>MHHHHHHGSDDDDKRPEAKSAQPADGWKGERPRSEEDNELNLPNLAAAYSSILSSLGENPQRQGLLKTPWRAASAMQFFTKGYQETISDVLNDAIFDEDHDEMVIVKDIDMFSMCEHHLVPFVGKVHIGYLPNKQ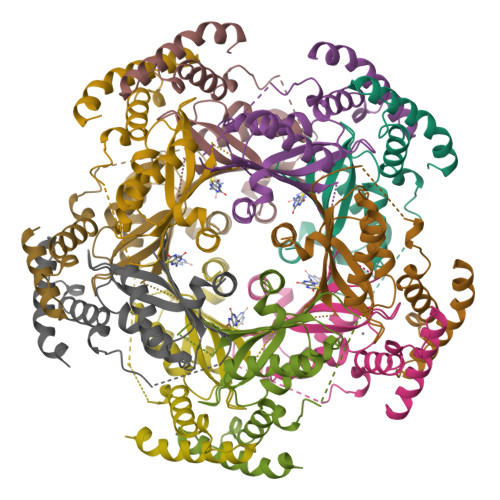VLGLSKLARIVEIYSRRLQVQERLTKQIAVAITEALRPAGVGVVVEATHMCMVMRGVQKMNSKTVTSTMLGVFREDPKTREEFLTLIRS[10x]>[2x]TSPSSPPAFRLETSDGGQDGAEVDKAQLGYGAGPPPMESRFQDEDRNFPPQIKVNLNYRKGAGASQPDLNRFDRDRLFNVVARGNPEDLAGLLEYLRRTSKYLTDSEYTEGSTGKTCLMKAVLNLQDGVNACIQPLLEIDRDSGNPQPLVNAQCTDEYYRGHSALHIAIEKRSLQCVKLLVENGANVHAKACGHFFQKNQDTCFYFGELPLSLAACTKQWDVVNYLLENPHQPASLQAQDSLGNTVLHALVMIADDSAENSALVVRMYDGLLQAGARLCPN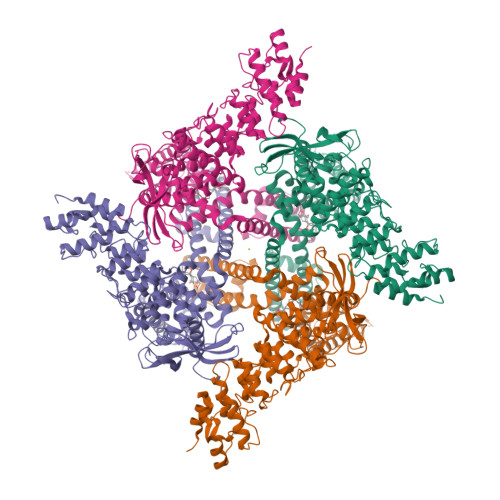VQLEGIPNLEGLTPLKLAAKEGKIEIFKHILQREFSAPCQSLSRKFTEWCYGPVRVSLYDLASVDSWEENSVLEIIAFHSRSPHRHRMVVLEPLNKLLQAKWDRLIPRFCFNFLCYLVYMLIFTAVAYHQPALEKQGFPPLKATAGNSMLLLGHILILLGGVYLLLGQLWYFWRRRLFIWISFMDSYSEILFLLQALLTVLSQVLCFLAIEWYLPLLVSSLVMGWTNLLYYTRGFQHTGIYSVMIEKVILRDLLRFLLVYLVFLFGFAVALVSLSREAQNSRTPAGPNATEVGQPGAGQEDEAPPYRSILDASLELFKFTIGMGELAFQEQLRFRGVVLLLLLAYVLLTYVLLLNMLIALMSETVNSVATDSWSIWKLQKAISVLEMENGYWWCRRKKQRAGVMLTVGTRPDGSPDERWCFRVGEMNWATWEQTLPRTLCEEPSGAAAPGVMKNPTPASQRGEDSASEEDHLPLQLLQSRDYKDDDDKAHHHHHH Clamp loaders are pentameric ATPases that place circular sliding clamps onto DNA, where they function in DNA replication and genome integrity. Because the sliding clamp is a closed ring in solution, it needs to be opened and placed onto DNA by a separate ATPase complex called the clamp loader. All clamp loaders are pentameric ATPases of the AAA + family (ATPases associated with various cellular activities). Here we describe a series of structures of the E. coli clamp loader in the process of placing the clamp onto a p/t-junction.

The dataset using the DNA-primed p/t-junction resulted in four conformations of the ternary complex after 3D classification. The first two are open states that differ in their collar domains (Open-DNAp/t and Altered-Collar), while the latter two are closed states that differ in their interactions between the loader and the clamp (Closed-DNA1 and Closed-DNA2). We first discuss the next on-pathway state where p/t-DNA binds inside the clamp loader and clamp, causing both to constrict around DNA. The primary motion is the pivoting of the A and B subunits out-of-plane into a spiral. The AAA+ modules of the γ-complex and the sliding clamp adopt a helical arrangement that matches the helical symmetry of DNA, similar to other structures of clamp loaders bound to p/t-DNA. This constriction results in the A-gate closing by ∼5 Å, measured by the centers of mass of domains A and E. The clamp then closes slightly, by 11 Å. Clamp closure is primarily driven by the relaxation of ß-clamp subunit I into a conformation that is more like that of the closed form (Cα-RMSDFully-Open_versus_Closed ∼3.3 Å versus Cα-RMSDDNA-Open_versus_Closed ∼1.8 Å). The Cα RMSD between the Open-RNAp/t structure and that of the Open-DNAp/t is only ∼0.7 Å. Both structures show that the duplex region of the p/t-junction adopts A-form geometry as expected. Because double-stranded DNA prefers B-form geometry in solution, it must be converted to A-form upon binding in the central chamber. On the other hand, trans-acting lysines (γ Lys141 and δ′ Lys130) directly contact the Walker B motif (Asp126) of the neighboring ATPase active site only after p/t-junction binding.

> MIRLYPEQLRAQLNEGLRAAYLLLGNDPLLLQESQDAVRQVAAAQGFEEHHTFSIDPNTDWNAIFSLCQAMSLFASRQTLLLLLPENGPNAAINEQLLTLTGLLHDDLLLIVRGNKLSKAQENAAWFTALANRSVQVTCQTPEQAQLPRWVAARAKQLNLELDDAANQVLCYCYEGNLLALAQALERLSLLWPDGKLTLPRVEQAVNDAAHFTPFHWVDALLMGKSKRALHILQQLRLEGSEPVILLRTLQRELLLLVNLKRQSAHTPLRALFDKHRVWQNRRGMMGEALNRLSQTQLRQAVQLLTRTELTLKQDYGQSVWAELEGLSLLLCHKPLADVFIDG;>[3x]GPHMSYQVLARKWRPQTFADVVGQEHVLTALANGLSLGRIHHAYLFSGTRGVGKTSIARLLAKGLNCETGITATPCGVCDNCREIEQGRFVDLIEIDAASRTKVEDTRDLLDNVQYAPARGRFKVYLIDEVHMLSRHSFNALLKTLEEPPEHVKFLLATTDPQKLPVTILSRCLQFHLKALDVEQIRHQLEHILNEEHIAHEPRALQLLARAAEGSLRDALSLTDQAIASGDGQVSTQAVSAMLGTLDDDQALSLVEAMVEANGERVMALINEAAARGIEWEALLVEMLGLLHRIAMVQLSPAALGNDMAAIELRMRELARTIPPTDIQLYYQTLLIGRKELPYAPDRRMGVEMTLLRALAFHPRMPLPEPEVPRQ;> GPHMRWYPWLRPDFEKLVASYQAGRGHHALLIQALPGMGDDALIYALSRYLLCQQPQGHKSCGHCRGCQLMQAGTHPDYYTLAPEKGKNTLGVDAVREVTEKLNEHARLGGAKVVWVTDAALLTDAAANALLKTLEEPPAETWFFLATREPERLLATLRSRCRLHYLAPPPEQYAVTWLSREVTMSQDALLAALRLSAGSPGAALALFQGDNWQARETLCQALAYSVPSGDWYSLLAALNHEQAPARLHWLATLLMDALKRHHGAAQVTNVDVPGLVAELANHLSPSRLQAILGDVCHIREQLMSVTGINRELLITDLLLRIEHYLQPGVVLPVPHL;>GPHMKFTVEREHLLKPLQQVSGPLGGRPTLPILGNLLLQVADGTLSLTGTDLEMEMVARVALVQPHEPGATTVPARKFFDICRGLPEGAEIAVQLEGERMLVRSGRSRFSLSTLPAADFPNLDDWQSEVEFTLPQATMKRLIEATQFSMAHQDVRYYLNGMLFETEGEELRTVATDGHRLAVCSMPIGQSLPSHSVIVPRKGVIELMRMLDGGDNPLRVQIGSNNIRAHVGDFIFTSKLVDGRFPDYRRVLPKNPDKHLEAGCDLLKQAFARAAILSNEKFRGVRLYVSENQLKITANNPEQEEAEEILDVTYSGAEMEIGFNVSYVLDVLNALKCENVRMMLTDSVSSVQIEDAASQSAAYVVMPMRL[2x]> MHHHHHHAVRASEISRVYEAYPEKKATLY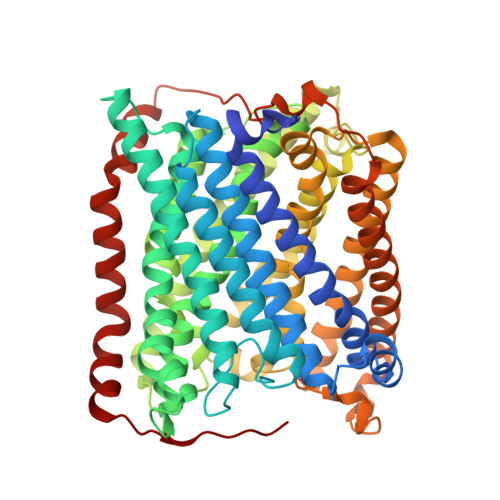FLVLGFLALIVGSLFGPFQALNYGNVDAYPLLKRLLPFVQSYYQGLTLHGVLNAIVFTQLFAQAIMVYLPARELNMRPNMGLMWLSWWMAFIGLVVAALPLLANEATVLYTFYPPLKGHWAFYLGASVFVLSTWVSIYIVLDLWRRWKAANPGKVTPLVTYMAVVFWLMWFLASLGLVLEAVLFLLPWSFGLVEGVDPLVARTLFWWTGHPIVYFWLLPAYAIIYTILPKQAGGRLVSDPMARLAFLLFLLLSTPVGFHHQFADPGIDPTWKMIHSVLTLFVAVPSLMTAFTVAASLEFAGRLRGGRGLFGWIRALPWDNPAFVAPVLGLLGFIPGGAGGIVNASFTLDYVVHNTAWVPGHFHLQVASLVTLTAMGSLYWLLPNLTGKPISDAQRRLGLAVVWLWFLGMMIMAVGLHWAGLLNVPRRAYIAQVPDAYPHAAVPMVFNVLAGIVLLVALLLFIYGLFSVLLSRERKPELAEAPLPFAEVISGPEDRRLVLAMDRIGFWFAVAAILVVLAYGPTLVQLFGHLNPVPGWRLW>GHRNLVRKSVRNLSPAERASLVAALKSLQEDSSADGFQSLASFHAQPPLCPAPAANKAFACCVHGMATFPEWHRLYTVQFEDALRRHGSVVGIPYWDTVVPQEDLPAFFNDEIWDDALFHANFTNPFNGADIDFNHQKIARDINVDKLAKEGPKGYDTWSFKQYIYALEQEDYCDFEVQFEIAHNAIHAWVGGTEEYSMGHLHYASYDPVFILHHSNTDRLFALWQELQKFRGHDPNEVNCALEMMREPLKPFSFGAPYNLNPTTKEHSKPEDTFDYKGHFHYEYDHLELQGMNVQRLHDYINQQKEADRVFAGFLLEGIGTSAHLDFSICAIDGECTHAGYFDVLGGSLETPWQFDRLYKYEIT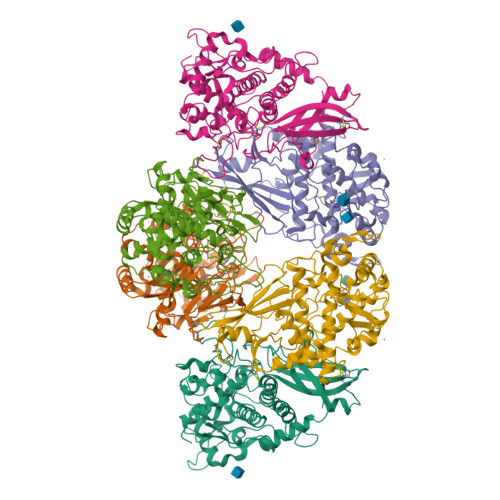DVLESKGLDVHDVFDIKITQTSWDNEDISTDRFPPPSVIYVPK[3x]>AMVSSLPKESQAELQLFQNEINAANPSDF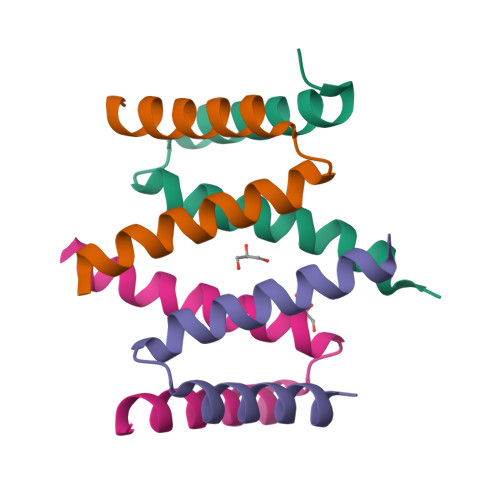LQFSANYFNKRLEQQRAFLKAR[8x]>[3x]G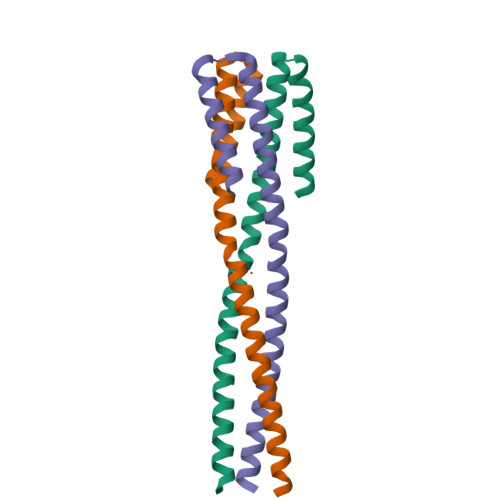SHMGTEDLKYSLERLREILERLEENPSEKQIVEAIRAIVENNAQIVEAIRAIVENNAQIVENNRAIIENNEAIGGGTKQLEEMKKQLKDLKRSLERG>MSLEKWRIYEELTNAVREFESINPVRLIPEVGTNFVYSLPLPYARSTKDVAGVKGRIVKYGNSVKAVGPVEFGASDHLARAVLTYMRFYPEYRSAINIRYSREIIEEIIEIAQERGFKVSFYDRREEPEEIKAKEGATIPWGIETAIKRIKERPDIIYHLGDVGKEPMILVFGRNPREVLEKIKMLIEGHHHHHH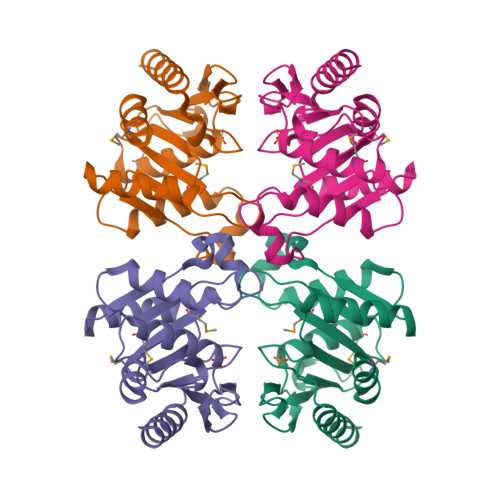[2x]> ANIVGGIEYSINNASLCSVGFSVTRGATKGFVTAGHCGTVNATARIGGAVVGTFAARVFPGNDRAWVSLTSAQTLLPRVANGSSFVTVRGSTEA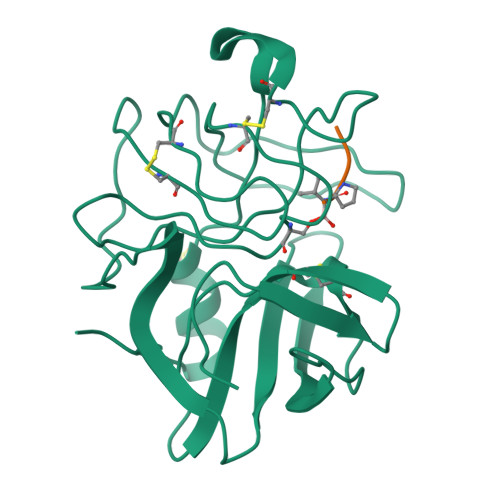AVGAAVCRSGRTTGYQCGTITAKNVTANYAEGAVRGLTQGNACMGRGDSGGSWITSAGQAQGVMSGGNVQSNGNNCGIPASQRSSLFERLQPILSQYGLSLVTG;> XAAPV>[2x]MSYIPGQPVTA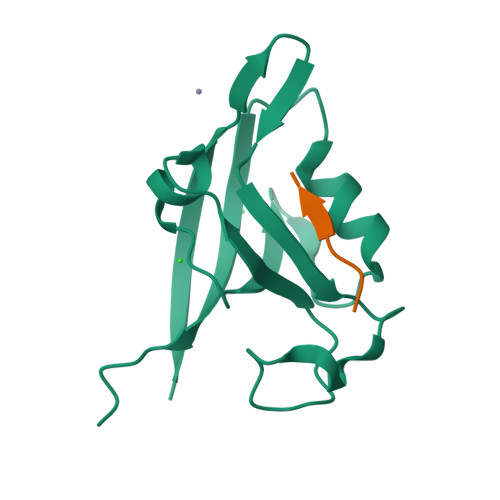VVQRVEIHKLRQGENLILGFSIGGGIDQDPSQNPFSEDKTDKGIYVTRVSEGGPAEIAGLQIGDKIMQVNGWDMTMVTHDQARKRLTKRSEEVVRLLVTRQSLQKAVQQSMLS;>NISYRRESAI[2x]> MGRLVLLWGAAVFLLGGWMALGQGGAAEGVQIQIIYFNLETVQVTWNASKYSRTNLTFHYRFNGDEAYDQCTNYLLQEGHTSGCLLDAEQRDDILYFSIRNGTHPVFTASRWMVYYLKPSSPKHVRFSWHQDAVTVTCSDLSYGDLLYEVQYRSPFDTEWQSKQENTCNVTIEGLDAEKCY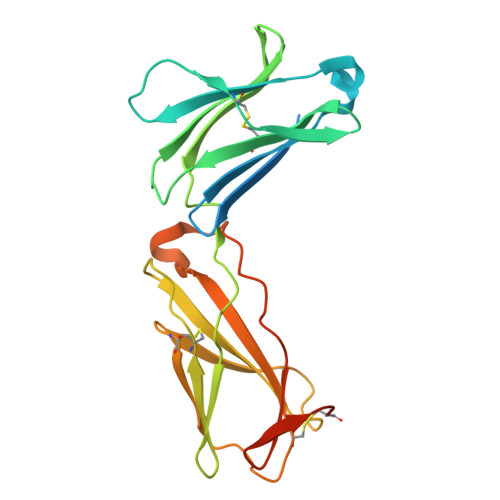SFWVRVKAMEDVYGPDTYPSDWSEVTCWQRGEIRDACAETGTKHHHHHH>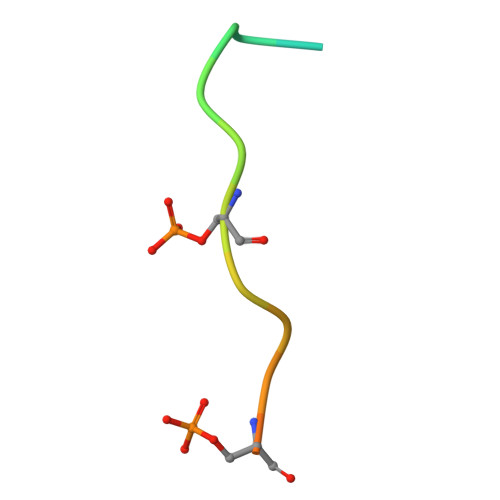 MTSPFNGLTSPQRSPFPKS>[4x]MRGSHHHHHHGSMEEYYMKLALDLAKQGEGQTESNPLVGAVVVKDGQIVGMGAHLKYGEAHAEVHAIHMAGAHAEGADIYVTLEPCSHYGKTPPCAELIINSGIKRVFVAMRDPNPLVAGRGISMMKEAGIEVREGILADQAERLNEKF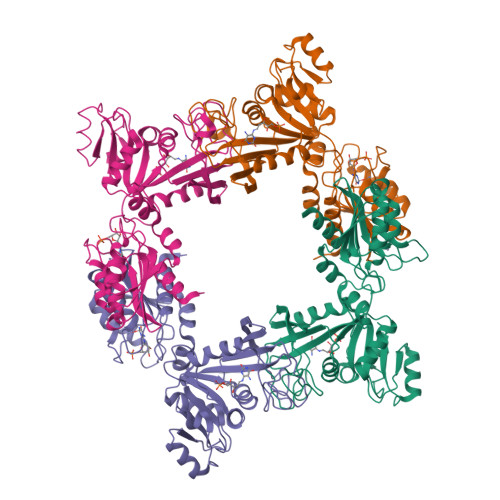LHFMRTGLPYVTLKAAASLDGKIATSTGDSKWITSEAARQDAQQYRKTHQSILVGVGTVKADNPSLTCRLPNVTKQPVRVILDTVLSIPEDAKVICDQIAPTWIFTTARADEEKKKRLSAFGVNIFTLETERIQIPDVLKILAEEGIMSVYVEGGSAVHGSFVKEGCFQEIIFYFAPKLIGGTHAPSLISGEGFQSMKDVPLLQFTDITQIGRDIKLTAKPTKE>[2x]HLTMPYVMPGDGEVVGVGEPVAIRFDENIADRGAAEKAIKITTNPPVEGAFYWLNNREVRWRPEHFWKPGTAVDVAVNTYGVDLGEGMFGEDNVQTHFTIGDEVIATADDNTKILTVRVNGEVVKSMPTSMGKDST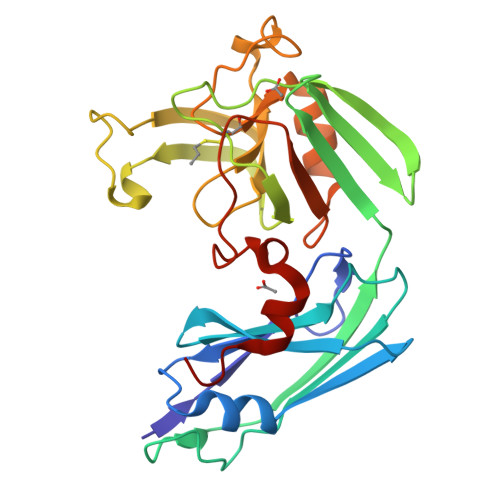PTANGIYIVGSRYKHIIMDSSTYGVPVNSPNGYRTDVDWATQISYSGVFVHSAPWSVGAQGHTNTSHGCLNVSPSNAQWFYDHVKRGDIVEVVNTVGGTLPGIDGLGDWNIPWDQWRAGNAKA> VPRGSHMKKLLVANRGEIAVRVFRACNELGLSTVAVYAREDEYSVHRFKADESYLIGQGKKPIDAYLDIDDIIRVALESGADAIHPGYG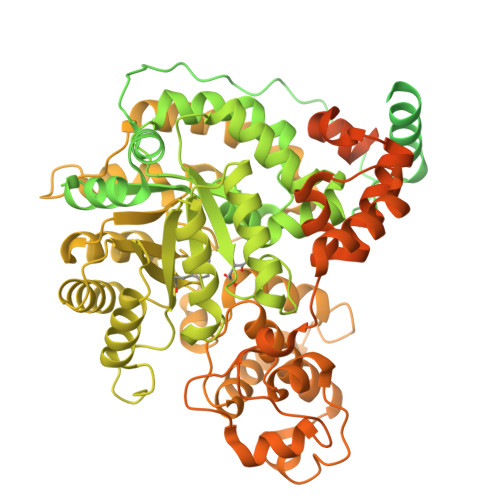LLSENLEFATKVRAAGLVFVGPELHHLDIFGDKIKAKAAADEAKVPGIPGTNGAVDIDGALEFAKTYGYPVMIKAALGGGGRGMRVARNDAEMHDGYARAKSEAIGAFGSGEIYVEKYIENPKHIEVQILGDRHGNIIHLHERDCSVQRRNQKVIEIAPAVGLSPDFRNEICEAAVKLCKNVGYVNAGTVEFLVKDDKFYFIEVNPRVQVEHTITELITGVDIVQAQILIAQGKDLHREIGLPAQSEIPLLGSAIQCRITTEDPQNGFLPDTGKIDTYRSPGGFGIRLDVGNAYAGYEVTPYFDSLLVKVCTFANEFSDSVRKMDRVLHEFRIRGVKTNIPFLINVIANENFTSGQATTTFIDNTPSLFNFPRLRDRGTKTLHYLSMITVNGFPGIENTEKRHFEEPRQPLLNLEKKKTAKNILDEQGADAVVDYVKNTKEVLLTDTTLRDAHQSLLATRLRLQDMKGIAQAIDQGLPELFSAEMWGGATFDVAYRFLNESPWYRLRKLRKLMPNTMFQMLFRGSNAVGYQNYPDNVIEEFIRVAAHEGIDVFRIFDSLNWLPQMEKSIQAVRDNGKIAEATICYTGDILDPSRPKYNIQYYKDLAKELEATGAHILAVKDMAGLLKPQAAYRLISELKDTVDLPIHLHTHDTSGNGIITYSGATQAGVDIIDVATASLAGGTSQPSMQSIYYALEHGPRHASINVKNAEQIDHYWEDVRKYYAPFEAGITSPQTEVYMHEMPGGQYTNLKSQAAAVGLGHRFDEIKQMYRKVNMMFGDIIKVTPSSKVVGDMALFMIQNDLTEEDVYARGNELNFPESVVSFFRGDLGQPVGGFPEKLQKIIVKDKAVITDRPGLHAEKVDFETVKADLEQKIGYEPGDHEVISYIMYPQVFLDYQKMQREFGAVTLLDTPTFLHGMRLNEKIEVQIEKGKTLSIRLDEIGEPDLAGNRVLFFNLNGQRREVVINDQSVQAQVVAKRKAETGNPNQIGATMPGSVLEILVKAGDKVQKGQALMVTEAMKMETTIEAPFDGEIVDLHVVKGEAIQTQDLLIEIN> ATRELDELMASLSDFKFMAQ;> SGRHERDAFDTLFDHAPDKLNVVKKTLITFVNKHLNKLNLEVTELETQFADGVYLVLLMGLLEGYFVPLHSFFLTPDSFEQKVLNVSFAFELMQDGGLEKPKPRPEDIVNCDL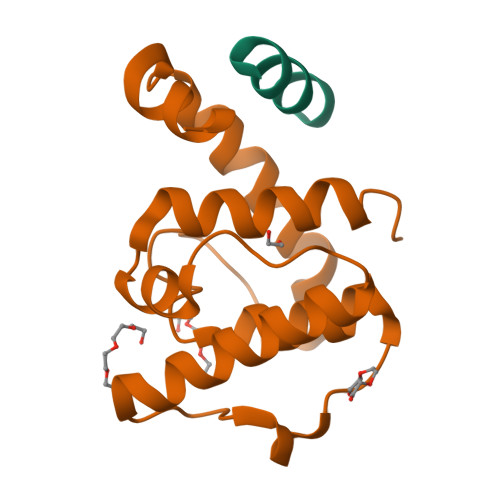KSTLRVLYNLFTKYRNVE>[2x]GSMKKERVITEFWDGKIIMVSPDDPKYALKKAEEVRELVDSELGFQQVSLRCPSQTRTYMFVSNEKKIVGCLIAEPIREAYRVLAEPPSLHSLHGEPLERHRAWRCSTEPEPAICGISRIWVFALMRRKAIASRMVDAVRSSFMYGSVLTTEEIAFSDPTPDGKLFASTYCKVPDFLVYNFVS;>[2x]VIGAKKA

Cohesin is loaded onto chromatin by the Scc2-Scc4 loader complex, however persistent cohesion cannot be established without the acetylation of two conserved tandem lysines on the Smc3 subunit by the Eco1 acetyltransferase (ACT). Eco1 is an acetyltransferase that belongs to the Gcn5-related N-acetyltransferase (GNAT) family. The xEco2 ACT fold is divided into two domains: the N-terminal domain contains α helix 1 and 2, and β strand 1–5 with a conserved central β hairpin insertion between β4 and β5 that is unique to cohesin ACTs; the C-terminal domain contains α helix 3, and β strand 6 and 7. The binding site for CoA is sandwiched between the N- and C-terminal domains involving β5 and α3, while the substrate peptides binds mainly to the central β hairpin and the C-terminal domain including the conserved C-terminal extension (C extension).

To circumvent this problem, we exploited the strong binding of CoA to ACTs and synthesized two 13-residue Smc3 (residues 99–111) peptide-CoA conjugates (K105-CoA and K106-CoA) each containing an isopropionyl bridge: peptide K105-CoA is conjugated with CoA at K105 whereas peptide K106-CoA has CoA conjugated to K106. The xEco2-K105-CoA structure represents the faster acetylation event on S. cerevisiae K112 of Smc3. The peptide K105-CoA adopts a β turn conformation, which is readily accommodated by the substrate-binding site created by the extended loop connecting α1 to β3, the short loop connecting β6 to α3, the central β hairpin, and the C extension on the xEco2 structure. The side chain of K105-CoA, which protrudes from the CoA-binding cavity, is gated by the conserved L562 and F564 residues. The unmodified K106 salt-bridges to D677. This mode of coordinating K106 explains why a basic residue is favoured at P + 1 in the non-directional motif consensus. In addition, the conserved C extension of xEco2 forms a contiguous anti-parallel β sheet with residues 101–104 of the substrate hairpin, wherein I102 forms a hydrophobic contact with V701. In fact, surface calculation using the PISA server shows that xEco2 and the K105 peptide (excluding CoA) has a protein-protein interface of 260 Å2 versus 486 Å2 between xEco2 and the K106 peptide. The smaller protein-protein interface could translate to a faster substrate release and turnover of S. cerevisiae K112 acetylation as seen in MS and the weaker peptide density in xEco2-K105-CoA structure (compare Supplementary Fig. 4A and B). The requirement for substantial conformational changes of K106 substrate binding compared to the readily accommodated K105 substrate by xEco2 may also explain why K105 acetylation is a faster and more rapid event.> ETGSAKVAFSAIRSTNHEPSEMSNRTMIIYFDQVLVNIGNNFDSERSTFIAPRKGIYSFNFHVVKVYNRQTIQVSLMLNGWPVISAFAGDQDVTREAASNGVLIQMEKGDRAYLKLERGNLMGGWKYSTFSGFLVFPLGSELGSGSAKVAFSAIRSTNHEPSEMSNRTMIIYFDQVLVNIGNNFDSERSTFIAPRKGIYSFNFHVVKVYNRQTIQVSLMLNGWPVISAFAGDQDVTREAASNGVLIQMEKGDRAYLKLERGNLMGGWKYSTFSGFLVFPLGSASGSGSAKVAFSAIRSTNHEPSEMSNRTMIIYFDQVLVNIGNNFDSERSTFIAPRKGIYSFNFHVVKVYNRQTIQVSLMLNGWPVISAFAGDQDVTREAASNGVLIQMEKGDRAYLKLERGNLMGGWKYSTFSGFLVFPLGTGGSGGSGGSGGSGGSGGSGGSGGSGGSGGSDSIIHIGAIFDESAKKDDEVFRTAVGDLNQNEEILQ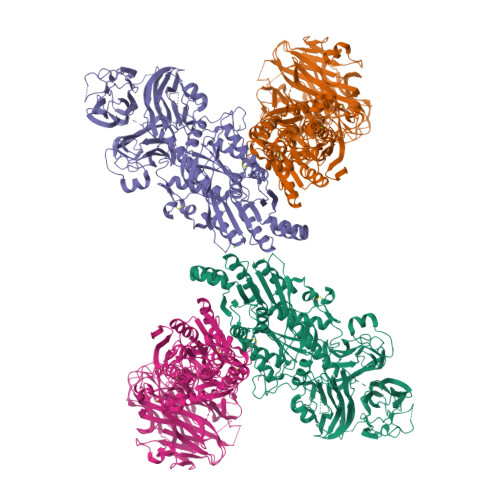TEKITFSVTFVDGNNPFQAVQEACELMNQGILALVSSIGCTSAGSLQSLADAMHIPHLFIQRSTAGTPRSGCGLTRSNRNDDYTLSVRPPVYLHDVILRVVTEYAWQKFIIFYDSEYDIRGIQEFLDKVSQQGMDVALQKVENNINKMITTLFDTMRIEELNRYRDTLRRAILVMNPATAKSFITEVVETNLVAFDCHWIIINEEINDVDVQELVRRSIGRLTIIRQTFPVPQNISQRCFRGNHRISSTLCDPKDPFAQNMEISNLYIYDTVLLLANAFHKKLEDRKWHSMASLSCIRKNSKPWQGGRSMLETIKKGGVSGLTGELEFGENGGNPNVHFEILGTNYGEELGRGVRKLGCWNPVTGLNGSLTDKKLENNMRGKHHHHHH> MGSMHQQHSKSENKPQQQRKKFEGPKREAILDLAKYKDSKIRVKLMGGKLVIGVLKGYDQLMNLVLDDTVEYM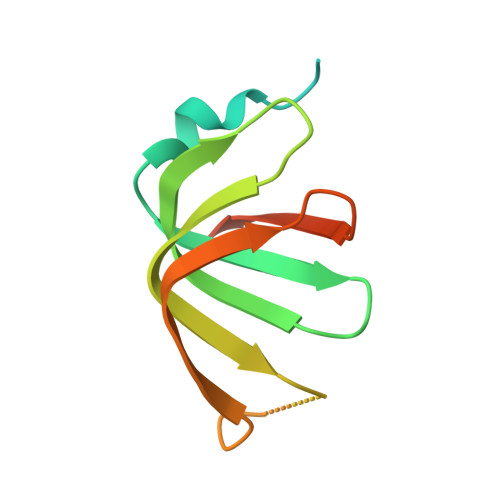SNPDDENNTELISKNARKLGLTVIRGTILVSLSSAEGSDVLYMQK> GMTDGEAVSAAAGPGAEGPPGPVGHWAPGSHILWRYRENGGPHVHIARPVTVVRDDADLLAVWLAPGTECVKPVLADGTPVHLEPLATRYTKPRTVQRDQWFGTGVLKLARPGEAWSVWLFWDPGWRF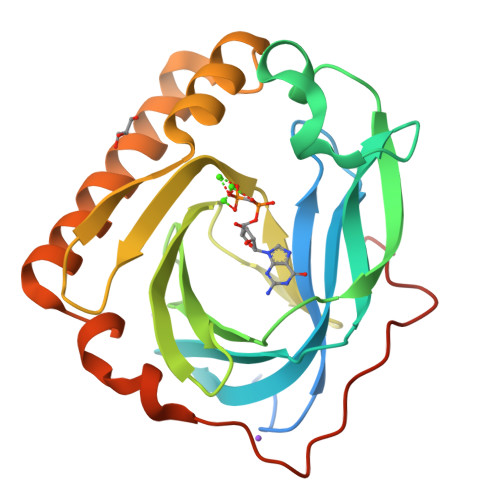KNWYVNLERPLTRWEGGVDSEDHFLDISVHPDRTWHWRDEDEFAQALRDGLMDPASAGRVRRAGRSAVAEIRAWGSPFADGWEHWRPDPAWPVPSLPGDWDRTPAHVSS(5E,17R,20S)-23-amino-20-hydroxy-14,20-dioxo-15,19,21-trioxa-20lambda~5~-phosphatricos-5-en-17-yl hexadecanoate | C35 H68 N O8 P | 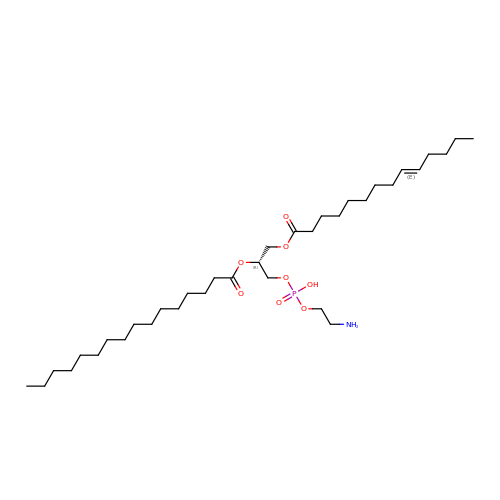IXIBEFBSXYIWMP-VCRBCDDQSA-N> MVVTRIAPSPTGDPHVGTAYIALFNYAWARRNGGRFIVRIEDTDRARYVPGAEERILAALKWLGLSYDEGPDVGGPHGPYRQSERLPLYQKYAEELLKRGWAYRAFETPEELEQIRKEKGGYDGRARNIPPEEAEERARRGEPHVIRLKVPRPGTTEVKDELRGVVVYDNQEIPDVVLLKSDGYPTYHLANVVDDHLMGVTDVIRAEEWLVSTPIHVLLYRAFGWEAPRFYHMPLLRNPDKTKISKRKSHTSLDWYKAEGFLPEALRNYLCLMGFSMPDGREIFTLEEFIQAFTWERVSLGGPVFDLEKLRWMNGKYIREVLSLEEVAERVKPFLREAGLSWESEAYLRRAVELMRPRFDTLKEFPEKARYLFTEDYPVSEKAQRKLEEGLPLLKELYPRLRAQEEWTEAALE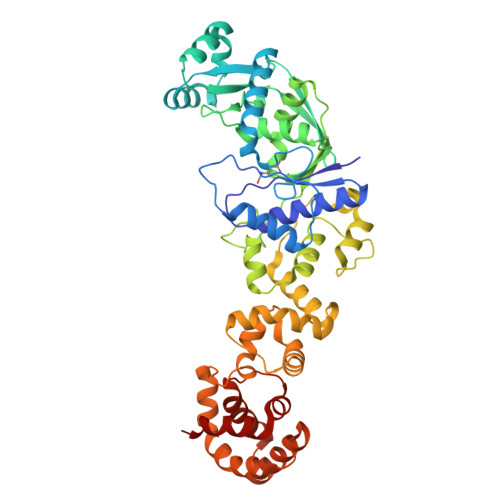ALLRGFAAEKGVKLGQVAQPLRAALTGSLETPGLFEILALLGKERALRRLERALA> HGSPVDICTAKPRDIPMNPMCIYRSPEKKATEDEGSEQKIPEATNRRVWELSKANSRFATTFYQHLADSKNDNDNIFLSPLSISTAFAMTKLGACNDTLQQLMEVFKFDTISEKTSDQIHFFFAKLNCRLYRKAQKSSKLVSAN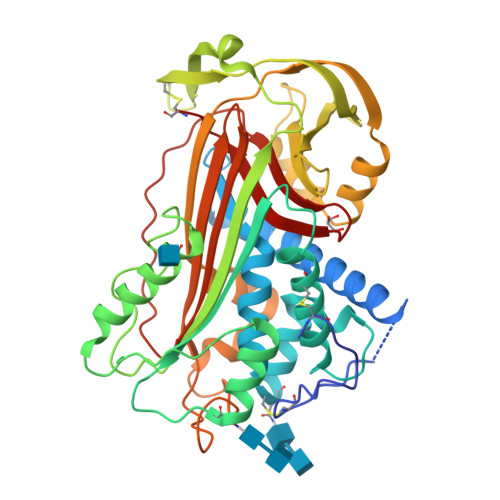RLFGDKSLTFNETYQDISELVYGAKLQPLDFKENAEQSRAAINKWVSNKTEGRITDVIPSEAINELTVLVLVNTIYFKGLWKSKFSPENTRKELFYKADGESCSASMMYQEGKFRYRRVAEGTQVLELPFKGDDITMVLILPKPEKSLAKVEKELTPEVLQEWLDELEEMMLVVHMPRFRIEDGFSLKEQLQDMGLVDLFSPEKSKLPGIVAEGRDDLYVSDAFHKAFLEVNEEGCEAAASTAVVIAGRSLNPNRVTFKANRPFLVFIREVPLNTIIFMGRVANPCVK;> HGSPVDICTAKPRDIPMNPMCIYRSPEKKATEDEGSEQKIPEATNRRVWELSKANSRFATTFYQHLADSKNDNDNIFLSPLSISTAFAMTKLGACNDTLQQLMEVFKFDTISEKTSDQIHFFFAKLNCRLYRKANKSSKLVSANRLFGDKSLTFNETYQDISELVYGAKLQPLDFKENAEQSRAAINKWVSNKTEGRITDVIPSEAINELTVLVLVNTIYFKGLWKSKFSPENTRKELFYKADGESCSASMMYQEGKFRYRRVAEGTQVLELPFKGDDITMVLILPKPEKSLAKVEKELTPEVLQEWLDELEEMMLVVHMPRFRIEDGFSLKEQLQDMGLVDLFSPEKSKLPGIVAEGRDDLYVSDAFHKAFLEVNEEGSEAAASTAVVIAGRSLNPNRVTFKANRPFLVFIREVPLNTIIFMGRVANPCVK> GSHMDYLVTEEEINLTRGPSGLGFNIVGGTDQQYVSNDSGIYVSRIKENGAAALDGRLQEGDKILSVNGQDLKNLLHQDAVDLFRNAGYAVSLRVQHRLQVQGSAYGSVKAYTNFDAERDALNIETAIKTKGVDEVTIVNILTNRSNEQRQDIAFAYQRRTKKELASALKSALSGHLETVILGLLKTPAQYDASELKASMKGLGTDEDSLIEIICSRTNQELQEINRVYKEMYKTDLEKDIISDTSGDFRKLMVALAKGRRAEDGSVIDYELI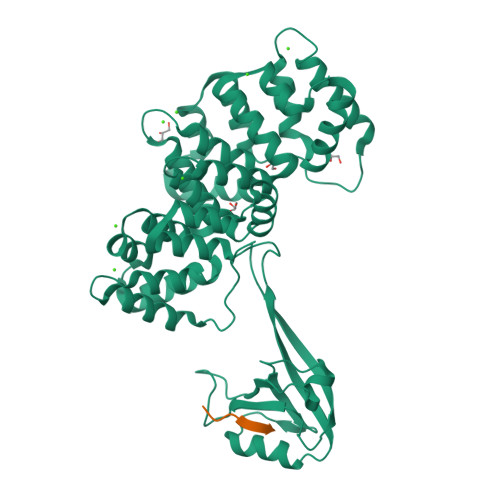DQDARDLYDAGVKRKGTDVPKWISIMTERSVPHLQKVFDRYKSYSPYDMLESIRKEVKGDLENAFLNLVQCIQNKPLYFADRLYDSMKGKGTRDKVLIRIMVSRSEVDMLKIRSEFKRKYGKSLYYYIQQDTKGDYQKALLYLCGGDD;> TDDSEKHFRETEV> MNDIAHNLAQVRDKISAAATRCGRSPEEITLLAVSATKPASAIAEAIDAGQRQFGENYVQEGVDKIRHFQELGVTGLEWHFIGPLQSNKSRLVAEHFDWCHTIDRLRIATRLNDQRPAELPPLNVLIQINISDENSASGIQLAELDELAAAVAELPRLRLR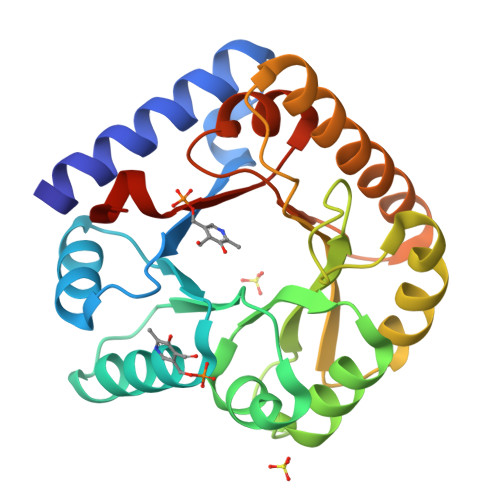GLMAIPAPESEYVRQFEVARQMAVAFAGLKTRYPHIDTLSLGMSDDMEAAIAAGSTMVRIGTAIFGARDYSKK>SEDRDTARVLLIMVRSLLKIGNPEDAEEVVKMIEELARRTND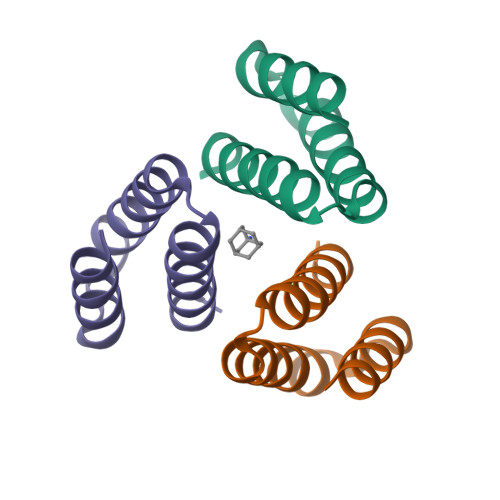PEIRRLLEEARKLVK[3x]ATAs transfer an amino group of a chiral amine compound to a ketone compound using the cofactor pyridoxal 5’-phosphate (PLP) with a high turnover rate, stable catalytic activity, broad substrate specificity and excellent stereoselectivity, which is achieved by a proposed large-binding pocket (L pocket) and small-binding pocket (S pocket) in the substrate-binding site8910111213141516. Each protomer (subunit) of the dimeric enzymes shows a structural architecture typical of the fold-type IV class of PLP-dependent enzymes, which are made up of two domains. The substrate-binding site is surrounded by the cavity among the two domains, the cofactor PLP, and the loop consisting of the residues 129–145 of the other protomer. The substrate-binding site can be divided into two parts as described initially, the L pocket and the S pocket, which is consistent with the previously proposed mechanism for the substrate specificity of ATAs in which the smaller and larger atomic groups of substrates are recognized by the S and L pockets, respectively.

The G136F mutant was derived from structural comparison between Ab-R-ATA and ATA-117-Rd11, where the 136th residue was considered as the main cause of the structural alteration of the loop near the active site as will be described. The loops 129–145 of the G136F mutant and ATA-117-Rd11 showed significantly different conformation from that of the wild-type, depending on the amino acid residue at the position 136. Gly136 was located near Val152 in the wild-type, whereas Phe136 was distant from Val152 in the G136F mutant and ATA-117-Rd11, accompanied by the long-range alteration of the loop’s backbone conformation. This suggests that the probable steric hindrance between the bulky side chain of Phe136 and Val152 was the main cause of the conformational difference. The G136F/Y/H/W mutants show more than 40-fold lower kcat/Km values towards pyruvate, indicating that these mutants could not recognize pyruvate properly. This is probably due to the introduction of a bulky side chain into the residue 136, which could have altered the conformation of the loop 129–145, and thus caused Arg138, the key residue for pyruvate recognition, to move out from the active site. The alteration of the loop 129–145 varied the properties of the substrate binding site drastically. Simultaneously, Arg138 was moved away from the substrate-binding site by the alteration of the loop, resulting in an enlargement of the cavity to accommodate large substrates. These conclusions could well explain how the G136F/Y/H/W mutants favor bulky and hydrophobic substrates.

>MAFSADTSEIVYTHDTGLDYITYSDYELDPANPLAGGAAWIEGAFVPPSEARISIFDQGYLHSDVTYTVFHVWNGNAFRLDDHIERLFSNAESMRIIPPLTQDEVKEIALELVAKTELREAFVSVSITRGYSSTPFERDITKHRPQVYMYAVPYQWIVPFDRIRDGVHAMVAQSVRRTPRSSIDPQVKNFQWGDLIRAVQETHDRGFEAPLLLDGDGLLAEGSGFNVVVIKDGVVRSPGRAALPGITRKTVLEIAESLGHEAILADITLAELLDADEVLGCTTAGGVWPFVSVDGNPISDGVPGPITQSIIRRYWELNVESSSLLTPVQY[12x]> METQLQSIFEEVVKTEVIEEAFPGMFMDTPEDEKTKLISCLGAFRQFWGGLSQESHEQCIQWIVKFIHGQHSPKRISFLYDCLAMAVETGLLPPRLVCESLINSDTLEWERTQLWALTFKLVRKIIGGVDYKGVRDLLKVILEKILTIPNTVSSAVVQQLLAAREVIAYILERNACLLPAYFAVTEIRKLYPEGKLPHWLLGNLVSDFVDTFRPTARINSICGRCSLLPVVNNSGAICNSWKLDPATLRFPLKGLLPYDKDLFEPQTALLRYVLEQPYSRDMVCNMLGLNKQHKQRCPVLEDQLVDLVVYAMERSETEEKFDDGGTSQLLWQHLSSQLIFFVLFQFASFPHMVLSLHQKLAGRGLIKGRDHLMWVLLQFISGSIQKNALADFLPVMKLFDLLYPEKEYIPVPDINKPQSTHAFAMTCIWIHLNRKAQNDNSKLQIPIPHSLRLHHEFLQQSLRNKSLQMNDYKIALLCNAYSTNSECFTLPMGALVETIYGNGIMRIPLPGTNCMASGSITPLPMNLLDSLTVHAKMSLIHSIATRVIKLAHAKSSVALAPALVETYSRLLVYMEIESLGIKGFISQLLPTVFKSHAWGILHTLLEMFSYRMHHIQPHYRVQLLSHLHTLAAVAQTNQNQLHLCVESTALRLITALGSSEVQPQFTRFLSDPKTVLSAESEELNRALILTLARATHVTDFFTGSDSIQGTWCKDILQTIMSFTPHNWASHTLSCFPGPLQAFFKQNNVPQESRFNLKKNVEEEYRKWKSMSNENDIITHFSMQGSPPLFLCLLWKMLLETDHINQIGYRVLERIGARALVAHVRTFADFLVYEFSTSAGGQQLNKCIEILNDMVWKYNIVTLDRLILCLAMRSHEGNEAQVCYFIIQLLLLKPNDFRNRVSDFVKENSPEHWLQNDWHTKHMNYHKKYPEKLYFEGLAEQVDPPVQIQSPYLPIYFGNVCLRFLPVFDIVIHRFLELLPVSKSLETLLDHLGGLYKFHDRPVTYLYNTLHYYEMHLRDRAFLKRKLVHAIIGSLKDNRPQGWCLSDTYLKCAMNAREENPWVPDDTYYCRLIGRLVDTMAGKSPGPFPNCDWRFNEFPNPAAHALHVTCVELMALAVSGKEVGN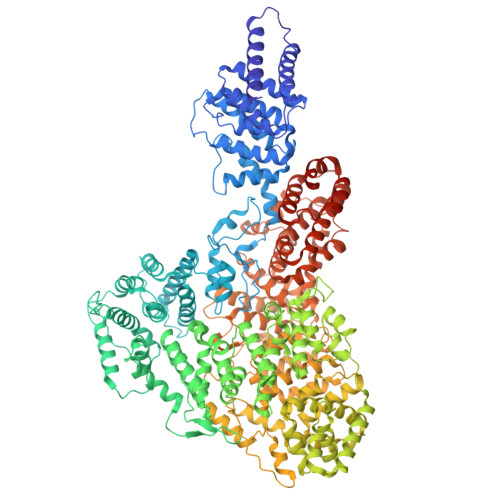ALLNVVLKSQPLVPRENITAWMNAIGLIITALPEPYWIVLHDRIVSVISSPSLTSETEWVGYPFRLFDFTACHQSYSEMSCSYTLALAHAVWHHSSIGQLSLIPKFLTEVLLPIVKTEFQLLYVYHLVGPFLQRFQQERTRCMIEIGVAFYDMLLNVDQCSTHLNYMDPICDFLYHMKYMFTGDSVKEQVEKIICNLKPALKLRLRFITHISKMEPAAVPPQAMNSGSPAPQSNQVPVSLPVTQ> MIRLPLLPTVIKNLFKKPATNPFPKTEPVPVPE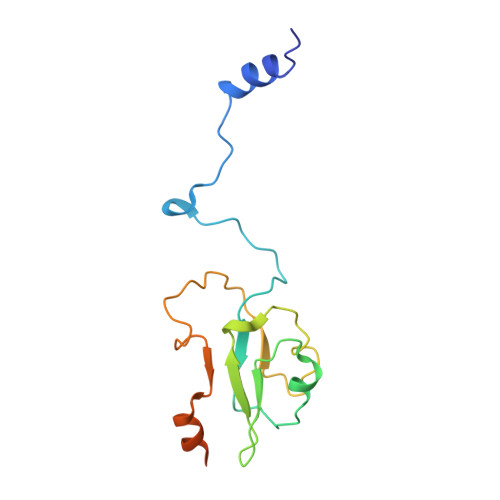DFRGKLVYNVDKCVGCRMCVTVCPAGVFVYLPEIRKVTLWIGRCVMCKQCVDVCPTAALQMSDEFLLASYDKYDAKLIYLTPEEAEDIKKKLEEANKAKAEKQASK>[2x]MGSSLRPLYMDVQATTPLDPRVLDAMLPYLINYYGNPHSRTHAYGWESEAAMERARQQVASLIGADPREIIFTSGATESNNIAIKGVARFYRSRKKHLITTQTEHKCVLDSCRSLEAEGFQVTYLPVQKSGIIDLKELEAAIQPDTSLVSVMTVNNEIGVKQPIAEIGRICSSRKVYFHTDAAQAVGKIPLDVNDMKIDLMSISGHKIYGPKGVGAIYIRRRPRVRVEALQSGGGQERGMRSGTVPTPLVVGLGAACEVAQQEMEYDHKRISKLSERLIQNIMKSLPDVVMNGDPKHHYPGCINLSFAYVEGESLLMALKDVALSSGSACTSASLEPSYVLRAIGTDEDLAHSSIRFGIGRFTTEEEVDYTVEKCIQHVKRLREMSPLWEMVQDGIDLKSIKWTQH;>MAASSRAQVLALYRAMLRESKRFSAYNYRTYAVRRIRDAFRENKNVKDPVEIQTLVNKAKRDLGVIRRQVHIGQLYSTDKLIIENRDMPRT[2x];>[2x]STIEERVKKIIGEQLGVKQEEVTNNASFVEDLGADSLDTVELVMALEEEFDTEIPDEEAEKITTVQAAIDYINGHQA;>[2x]MVLIDMSVDLSTQVVDHYENPRNVGSLDKTSKNVGTGLVGAPACGDVMKLQIQVDEKGKIVDARFKTFGCGSAIASSSLATEWVKGKTVEEALTIKNTDIAKELCLPPVKLHCSILAEDAIKAALADYKLKQEPKKGEAEKKELHHHHHH

Biogenesis involves the de novo synthesis of a Fe/S cluster on the scaffold protein ISCU, trafficking of the cluster via transient association to various targeting factors, and finally cluster insertion into specific recipient apoproteins. A critical initial step in Fe/S cluster synthesis is the supply of sulfur by the cysteine desulfurase NFS1. Here, we report crystal and solution structures of human NFS1 in association with ISD11-ACP, ISCU, FDX2, and FXN, together forming the ‘core ISC complex’. We show that eukaryote-specific ISD11 binds to NFS1 distal from the desulfurase active site and does not directly participate in catalysis.

Crystals obtained from purifications in the presence of ethylenediaminetetraacetic acid (EDTA) (termed (NIAU)2) did not contain divalent ions and diffracted to 3.15 Å, while those from purifications without EDTA contained a Zn ion bound between NFS1 and ISCU ((NIAU-Zn)2) and diffracted to 3.3 Å. The catalytic site for Fe/S cluster synthesis is best defined by the (NIAU-Zn)2 crystal structure showing a zinc bound to the persulfide-carrier Cys381 of the swung-out NFS1 Cys-loop and to putative ligands for de novo [2Fe–2S] cluster synthesis on the ISCU scaffold protein. The Zn site shows ~ 71% (chain D) and ~57% (chain H) occupancy in the two independent ISCU molecules. Importantly, the presence of Zn causes a reorientation of the Ala-loop of ISCU, with Cys44 approaching and facing the Zn ion, whereas Cys113 as part of helix α4 maintains its location most distant to the Zn ion. However, equivalent cysteine, aspartate, and histidine residues surround a [2Fe–2S] cluster in the archaeal Archaeoglobus fulgidus IscS-IscU complex17 and Zn in our (NIAU-Zn)2 structure. Of these, Cys44 and Cys70 are closest to the approaching NFS1 Cys381, while Cys113, biochemically proposed as a persulfide acceptor from NFS129, is most distant and part of a fixed α-helix. Interestingly, both the electron-donating [2Fe–2S] cluster of CtFdx2 and the iron-binding helix α1 of CtYfh1 were located close to the Fe/S cluster biosynthetic center delineated by the Zn ion present in the (NIAU-Zn)2 complex. We conclude that both the NFS1 Cys-loop and the ISCU Ala-loop undergo substantial structural adaptation in response to NFS1-ISCU docking.> SNAMNLFTRHRNNIRLTTAGEKLLPYAETLMNTWQAARKEVAHSSRHNEFSIGASASLWECMLNGWLGTLYSAPYNLQFEARIAQRQSLVKQLHERQLDLLITTESPKMDELSSQLLGNFTLALYCASPAKNRNELNYLRLEWGPDFQQNEVGLIGSDDVPLLTTSSAELIYQQLSRLNGCCWLPARWAKEKHGLHTVMDSATLSRPLYAIWLQNSDKQAQIHEIL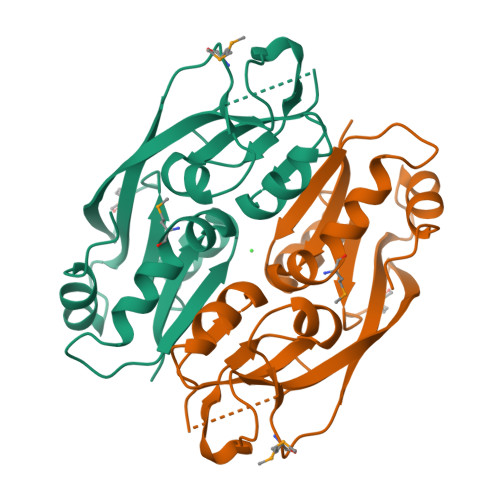KNPILE>GSSGSSGMASSCAVQVKLELGHRAQVRKKPTVEGFTHDWMVFVRGPEHSNIQHFVEKVVFHLHESFPRPKRVCKDPPYKVEESGYAGFILPIEVYFKNKEEPRKVRFDYDLFLHLEGHPPVNHLRCEKLTFNNPTEDFRRKLLKA[2x];>KGGKGLGKGG[2x]

Acetylated lysine (Kac) in the N-terminal tail of H3 or H4 provides a binding scaffold for reader proteins such as those containing a bromodomain or Yaf9, ENL, AF9, Taf14, and Sas5 (YEATS) domain. Another Kac-binding domain, the YEATS domain, consists of approximately 130 residues and forms an antiparallel β-sheet structure that can recognize and bind Kac and some acylated lysines. In humans, four YEATS domains are present in four different proteins (AF9, ENL, YEATS2, and GAS41). Human YEATS domains bind to the acetylated N-terminal tail of histone H3; however, their Kac-binding preferences at the level of the nucleosome are unknown.

We determined the crystal structures of AF9-YEATS complexed with the K5/K8- (1.95 Å resolution) and K8/K12- (2.00 Å resolution) diacetylated H4 peptides. The crystal forms of AF9-YEATS in complex with K5/K8- and K8/K12-diacetylated peptides both belonged to the space group P1, and each asymmetric unit contained two AF9-YEATS molecules (molecules A and B). Molecule A in complex with the H4K5ac/K8ac peptide (chain A) and molecules A and B in complex with two H4K8ac/K12ac peptides (chains A and B) recognized H4K8ac at the aromatic cage. The positively charged R61 and R64 residues of molecule B hydrogen bonded with chain A in both complexes. The electron density of H4K5ac was detected in the H4K5ac/K8ac peptide complex structure, but the position of the side chain of unmodified H4K5 in the H4K8ac/K12ac peptide complex could not be determined because of low electron density. K5ac and K12ac were located outside the aromatic cage; Nε of H4K5ac hydrogen bonded with E57 (left) and the added acetyl group of H4K12ac hydrogen bonded with D103 via a water molecule (right). The added acetyl group of H4K12ac interacted hydrophobically with H116 of AF9. The interaction modes of AF9-YEATS with H4K8ac and with H3K9ac were the same: the aromatic cage of AF9-YEATS hydrophobically interacted with the aromatic residues F28, H56, F59, Y78, and F81; and the amide and the carbonyl oxygen of the Kac side chain formed hydrogen bonds with the hydroxyl group of S58 and the backbone amide of Y78. The AF9-YEATS domain primarily recognized H4K8ac regardless of acetylation at K5 or K12. Therefore, the mode of primary binding to K8ac and secondary binding to K5ac or K12ac by the AF9-YEATS domain provides a unique molecular basis for sensing the hyperacetylation of H4 in the nucleus.> MHHHHHHSSRENLYFQGANSLSVHQLAAQGEMLYLATRIEQENVINHTDEEGFTPLMWAAAHGQIAVVEFLLQNGADPQLLGKGRESALSLACSKGYTDIVKMLLDCGVDVNEYDWNGGTPLLYAVHGNHVKCVKMLLESGADPTIE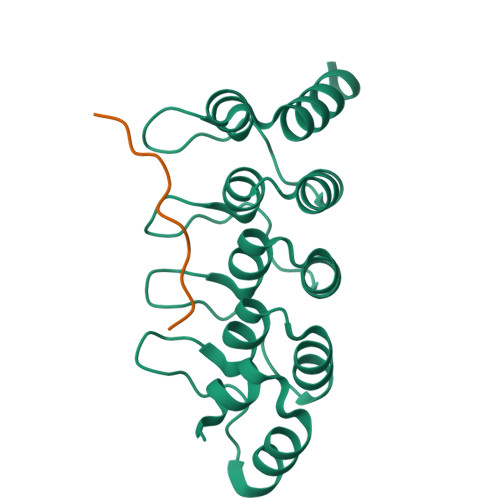TDSGYNSMDLAVALGYRSVQQVIESHLLKLLQNIKE;> HYRKTGSLLPTLPKLPSLS> II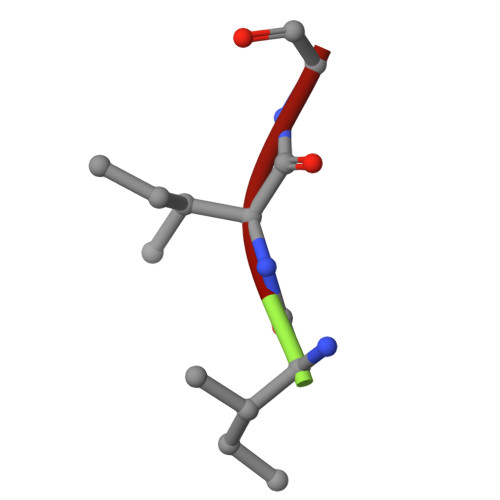G>[2x]MADPLTPAISDRICKHMNEDAASAIALYAQVFGQQTDVTMAQMQAIDPTGMDLVVESEGGSKTIRIEFEQPLKDSEDAHQVLIAMAKQARSVGKNSAENLYFQ

Using a phylogenomics-based approach and complementary structural techniques, we identify a family of dimeric hemoproteins comprising a domain of unknown function DUF2470. The heme iron is axially coordinated by two zinc-bound histidine residues, forming a distinct two-fold symmetric zinc-histidine-iron-histidine-zinc site. Together with structure-guided in vitro and in vivo experiments, we further demonstrate the existence of a functional link between heme binding by Dri1 (Domain related to iron 1, formerly ssr1698) and post-translational regulation of succinate dehydrogenase in the cyanobacterium Synechocystis, suggesting an iron-dependent regulatory link between photosynthesis and respiration. Given the ubiquity of proteins containing homologous domains and connections to heme metabolism across eukaryotes and prokaryotes, we propose that DRI (Domain Related to Iron; formerly DUF2470) functions at the molecular level as a heme-dependent regulatory domain. We heterologously expressed and purified the recombinant protein encoded by the Synechocystis gene dri1 (formerly known as ssr1698) and tested the heme-binding ability of this small, soluble protein (96 amino acids, 10 kDa).

His21Ala exhibits a shifted binding interface with a rotated heme ring (~34°) relative to WT Dri1. Calculated Polder OMIT maps with the heme, His residues, and bulk solvent excluded in addition to higher ligand B-factors reflect a loosely bound heme. The loss of His21, and presumably zinc binding, prevents axial ligation to the heme iron by His79. Instead, Asp20 seems most likely to be the side chain interacting with the heme iron, though the distance between the carboxyl functional group and iron is long (~4 Å Fe - O distance). This coordination distance can explain the increased heme rotation and mobility observed in MD simulations, resulting in a weaker bonding interaction and lower heme-binding ability. The His21Ala structure further suggests that zinc ions could bind via tetragonal ligation by His16, Asp20, Glu76, and His79 residues. However, since the Asp side chain can only have one binding interaction (as opposed to the two nitrogen sites in imidazole), zinc-binding might prevent Asp20 from interacting with the heme iron. Such a hypothesis is in line with the abrogation of heme binding by the addition of excess zinc to His21Ala. We observed that all variants with a single amino acid substitution retained heme binding to some extent. Both His21Ala and His21Ala-His79Ala variants displayed a red-shifted Soret peak at 415 nm, which corresponds to a reduced heme iron or a modified heme coordination.> SFDLRLYWTSLIADVEAELDAAMPIRTPERIHSAMRYAVLPGAGNEGTAKRAPPVLCVAACELLGAPREAALPAAVALEMLHAASLVHDDLPCFDAAPTRRGRPSTHAAYGTDMAVLAGDALFPLAYTHVIAHTPSPDPVPHAVLLRVLGELARAVGSTGMAAGQFLDLAGATALGEAEVMKVLTKKFGEMAECSAACGAMLGGAGPDEEAALRRYGRTIGVLYQLVDDIRSASGNGKMRSNASVLRALGMD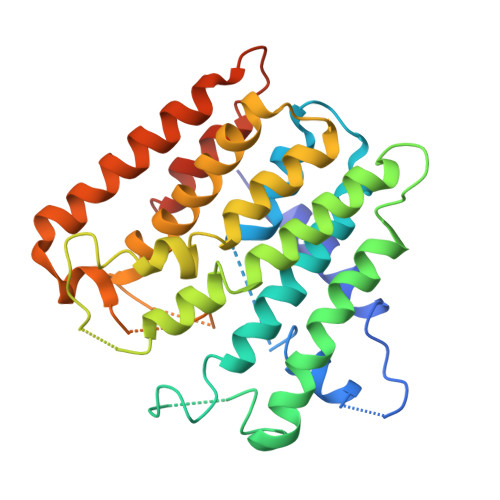RALGIVEELKAQAKMEADRFGDKYGERVLPLYSFVDYAVERGFELQDAATTP Complex I (NADH:ubiquinone (UQ) oxidoreductase) is the first and the largest enzyme of the respiratory chain, catalysing the transfer of two electrons from NADH to UQ, coupled to the translocation of four protons across the bacterial or inner mitochondrial membrane. In bacterial complex I the 14 “core” subunits, necessary and sufficient for complex I function, are shared equally between the peripheral and membrane arms, together forming an L-shaped molecule. All known co-factors of complex I reside in the PA: the primary electron acceptor flavin-mononucleotide (FMN) is connected by the redox chain of seven Fe–S clusters to the quinone-binding site (Q-site) at the interface with the membrane domain. In this work we address this question by building and analyzing atomic structures of nine different conformational states of complex I, which were obtained by X-ray crystallography and single-particle cryo-EM.

In contrast, binding of DQ substrate to Q-site, in the absence of NADH or NAD+ in the NADH-binding site, promotes the rotation and tilt of the entire PA, including subunits Nqo4 and Nqo6 near Q-site, correlated with concerted changes in the region of the nearest proton pump, the E-channel. This suggests that motions near the Q-site can lead to changes in the E-channel and can be driven just by DQ binding, without any redox reaction. Other key residues, such as H384 from the key β1–β2 loop (33-QHPSTHG-39) in Nqo4 and M516, also contribute to the stabilization of the quinone ring, while secondary residues are involved specifically in the binding of each ligand. In particular, DQ interacts mainly with the residues mentioned above with its hydrocarbon chain surrounded by hydrophobic residues that complete the stabilization of the entire ligand. The presence of DQ in the Q-site significantly alters the conformation of the Nqo4 β-sheet, pulling β1–β2 loop (residues 32–39) about 1.5 Å inside the cavity towards DQ, allowing for stacking interactions between H384 and DQ. The opposite Nqo6 β-sheet also shifts in a similar direction, but the strand flanking the Q-cavity (P386 to F416) remains in place, thus effectively moving into the cavity and narrowing it. Therefore, as a result of DQ binding, the entire Q cavity undergoes conformational changes so that it “tightens” significantly around the quinone headgroup. Strikingly, this coupling was the strongest in the CXIDQ structure, because it was augmented by an additional edge, extending from the Nqo6 subunit. Despite the overall similarity of water networks, we identified one notable difference: only in the CXIDQ structure we observe the presence of a single water molecule nested between E32 and E67 of Nqo11 subunit. Thus, placement of water in this position leads to the formation of a unique continuous path extending from Nqo11 to Nqo14, that is, a path connecting the E-channel and the first antiporter.

>[2x]MTGPILSGLDPRFERTLYAHVGKEGSWTLDYYLRHGGYETAKRVLKEKTPDEVIEEVKRSGLRGRGGAGFPTGLKWSFMPKDDGKQHYLICNADESEPGSFKDRYILEDVPHLLIEGMILAGYAIRATVGYIYVRGEYRRAADRLEQAIKEARARGYLGKNLFGTDFSFDLHVHRGAGAYICGEETALMNSLEGLRANPRLKPPFPAQSGLWGKPTTINNVETLASVVPIMERGADWFAQMGTEQSKGMKLYQISGPVKRPGVYELPMGTTFRELIYEWAGGPLEPIQAIIPGGSSTPPLPFTEEVLDTPMSYEHLQAKGSMLGTGGVILIPERVSMVDAMWNLTRFYAHESCGKCTPCREGVAGFMVNLFAKIGTGQGEEKDVENLEALLPLIEGRSFCPLADAAVWPVKGSLRHFKDQYLALAREKRPVPRPSLWR;>[2x]MGFFDDKQDFLEETFAKYPPEGRRAAIMPLLRRVQQEEGWIRPERIEEIARLVGTTPTEVMGVASFYSYYQFVPTGKYHLQVCATLSCKLAGAEELWDYLTETLGIGPGEVTPDGLFSVQKVECLGSCHTAPVIQVNDEPYVECVTRARLEALLAGLRAGKRLEEIELPGKCGHHVHEVEV;>[2x]MVRVKVNDRIVEVPPGTSVMDAVFHAGYDVPLFCSEKHLSPIGACRMCLVRIGLPKKGPDGKPLLNEKGEPEIQWQPKLAASCVTAVADGMVVDTLSDVVREAQAGMVEFTLLNHPLDCPTCDKGGACELQDRTVEYGLYEKYYQKGPLELPVYTRFEFTRRHVDKHHPLSPFVILDRERCIHCKRCVRYFEEVPGDEVLDFIERGVHTFIGTMDFGLPSGFSGNITDICPVGALLDLTARFRARNWEMEETPTTCALCPVGCGITADTRSGELLRIRAREVPEVNEIWICDAGRFGHEWADQNRLKTPLVRKEGRLVEATWEEAFLALKEGLKEARGEEVGLYLAHDATLEEGLLASELAKALKTPHLDFQGRTAAPASLFPPASLEDLLQADFALVLGDPTEEAPILHLRLSEFVRDLKPPHRYNHGTPFADLQIKERMPRRTDKMALFAPYRAPLMKWAAIHEVHRPGEEREILLALLGDKEGSEMVAKAKEAWEKAKNPVLILGAGVLQDTVAAERARLLAERKGAKVLAMTPAANARGLEAMGVLPGAKGASWDEPGALYAYYGFVPPEEALKGKRFVVMHLSHLHPLAERYAHVVLPAPTFYEKRGHLVNLEGRVLPLSPAPIENGEAEGALQVLALLAEALGVRPPFRLHLEAQKALKARKVPEAMGRLSFRLKELRPKERKGAFYLRPTMWKAHQAVGKAQEAARAELWAHPETARAEALPEGAQVAVETPFGRVEARVVHREDVPKGHLYLSALGPAAGLRVEGRVLVPAGGEA;>[2x]MREEFLEEIPLDAPPEEAKELRTEVMTLNVGPQHPSTHGVLRLMVTLSGEEVLEVVPHIGYLHTGFEKTMEHRTYLQNITYTPRMDYLHSFAHDLAYALAVEKLLGAVVPPRAETIRVILNELSRLASHLVFLGTGLLDLGALTPFFYAFRERETILDLFEWVTGQRFHHNYIRIGGVKEDLPEEFVPELKKLLEVLPHRIDEYEALFAESPIFYERARGVGVIPPEVAIDLGLTGGSLRASGVNYDVRKAYPYSGYETYTFDVPLGERGDVFDRMLVRIREMRESVKIIKQALERLEPGPVRDPNPQITPPPRHLLETSMEAVIYHFKHYTEGFHPPKGEVYVPTESARGELGYYIVSDGGSMPYRVKVRAPSFVNLQSLPYACKGEQVPDMVAIIASLDPVMGDVDR;>MRLERVLEEARAKGYPIEDNGLGNLWVVLPRERFKEEMAHYKAMGFNFLADIVGLDYLTYPDPRPERFAVVYELVSLPGWKDGDGSRFFVRVYVPEEDPRLPTVTDLWGSANFLEREVYDLFGIVFEGHPDLRKILTPEDLEGHPLRKDYPLGETPTLFREGRYIIPAEFRAALTGKDPGLTFYKGGSRKGYRSLWADLKKAREVKG[2x];>[2x]MALKDLFERDVQELEREGILFTTLEKLVAWGRSNSLWPATFGLACCAIEMMASTDARNDLARFGSEVFRASPRQADVMIVAGRLSKKMAPVMRRVWEQMPDPKWVISMGACASSGGMFNNYAIVQNVDSVVPVDVYVPGCPPRPEALIYAVMQLQKKVRGQAYNERGERLPPVAAWKRTRG;>[2x]MSASSERELYEAWVELLSWMREYAQAKGVRFEKEADFPDFIYRMERPYDLPTTIMTASLSDGLGEPFLLADVSPRHAKLKRIGLRLPRAHIHLHAHYEPGKGLVTGKIPLTKERFFALADRAREALAFA;>[2x]MTLKALAQSLGITLKYLFSKPVTVPYPDAPVALKPRFHGRHVLTRHPNGLEKCIGCSLCAAACPAYAIYVEPAENDPENPVSAGERYAKVYEINMLRCIFCGLCEEACPTGAIVLGYDFEMADYEYSDLVYGKEDMLVDVVGTKPQRREAKRTGKPVKVGYVVPYVRPELEGFKAPTEGGKR;>MAPIQEYVGTLIYVGVALFIGVAALLVGALLGPKKPGRAKLMPYESGNDPAGEVKRFPVHFYVVAMLFILFDVEVAFLWPYAVSAGGLGLYGFLGVLAFTLLLFVGFLYEWWKGVMRWH[2x];>MTWSYPVDPYWMVALKALLVVVGLLTAFAFMTLIERRLLARFQVRMGPNRVGPFGLLQPLADAIKSIFKEDIVVAQADRFLFVLAPLISVVFALLAFGLIPFGPPGSFFGYQPWVINLDLGILYLFAVSELAVYGIFLSGWASGSKYSLLGSLRSSASLISYELGLGLALLAPVLLVGSLNLNDIVNWQKEHGWLFLYAFPAFLVYLIASMAEAARTPFDLPEAEQELVGGYHTEYSSIKWALFQMAEYIHFITASALIPTLFLGGWTMPVLEVPYLWMFLKIAFFLFFFIWIRATWFRLRYDQLLRFGWGFLFPLALLWFLVTALVVALDLPRTYLLYLSALSFLVLLGAVLYTPKPARKGGGA[2x];>MSLLEGLALFLLLLSGVLVVTLRNAIHAALALILNFLVLAGVYVALDARFLGFIQVIVYAGAIVVLFLFVIMLLFAAQGEIGFDPLVRSRPLAALLALGVAGILAAGLWGLDLAFTQDLKGGLPQALGPLLYGDWLFVLLAVGFLLMAATVVAVALVEPGKASRAKEAEKREEVAR[2x];>MSYLLTSALLFALGVYGVLTRRTAILVFLSIELMLNAANLSLVGFARAYGLDGQVAALMVIAVAAAEVAVGLGLIVAIFRHRESTAVDDLSELRG[2x];>MALLGTILLPLLGFALLGLFGKRMREPLPGVLASGLVLASFLLGAGLLLSGGARFQAEWLPGIPFSLLLDNLSGFMLLIVTGVGFLIHVYAIGYMGGDPGYSRFFAYFNLFIAMMLTLVLADSYPVMFIGWEGVGLASFLLIGFWYKNPQYADSARKAFIVNRIGDLGFMLGMAILWALYGTLSISELKEAMEGPLKNPDLLALAGLLLFLGAVGKSAQIPLMVWLPDAMAGPTPVSALIHAATMVTAGVYLIARSSFLYSVLPDVSYAIAVVGLLTAAYGALSAFGQTDIKKIVAYSTISQLGYMFLAAGVGAYWVALFHVFTHAFFKALLFLASGSVIHALGGEQDVRKMGGLWKHLPQTRWHALIGALALGGLPLLSGFWSKDAILAATLTYPFGGVGFYVGALLVAVLTAMYAMRWFVLVFLGEERGHHHPHEAPPVMLWPNHLLALGSVLAGYLALPHPLPNVLEPFLKPALAEVEAHHLSLGAEWGLIALSAAVALLGLWAGFVFFQRKVFPAWYLAFEAASREAFYVDRAYNALIVNPLKALAEALFYGDRGLLSGYFGLGGAARSLGQGLARLQTGYLRVYALLFVLGALLLLGVMRW[2x];>[2x]MVVLAVLLPVVFGALLLLGLPRALGVLGAGLSFLLNLYLFLTHPGGVAHAFQAPLLPGAGVYWAFGLDGLSALFFLTIALTVFLGALVARVEGRFLGLALLMEGLLLGLFAARDLLVFYVFFEAALIPALLMLYLYGGEGRTRALYTFVLFTLVGSLPMLAAVLGARLLSGSPTFLLEDLLAHPLQEEAAFWVFLGFALAFAIKTPLFPLHAWLPPFHQENHPSGLADALGTLYKVGVFAFFRFAIPLAPEGFAQAQGLLLFLAALSALYGAWVAFAAKDFKTLLAYAGLSHMGVAALGVFSGTPEGAMGGLYLLAASGVYTGGLFLLAGRLYERTGTLEIGRYRGLAQSAPGLAALALILFLAMVGLPGLSGFPGEFLTLLGAYKASPWLAALAFLSVIASAAYALTAFQKTFWEEGGSGVKDLAGAEWGFALLSVLALLLMGVFPGYFARGLHPLAEAFAKLLGGGA;>[2x]MTLAILAVFSVALTLLGFVLPPQGVKRATLLGLALALASLLLTWGKPFAFGPYAVDGVSQVFTLLALLGALWTVGLVRSGRFEFYLLVLYAALGMHLLASTRHLLLMLVALEALSLPLYALATWRRGQGLEAALKYFLLGALAAAFFLYGAALFYGATGSLVLGAPGEGPLYALALGLLLVGLGFKAALAPFHFWTPDVYQGSPTPVVLFMATSVKAAAFAALLRVAAPPEALALLVALSVVVGNLAALAQKEAKRLLAYSSIAHAGYMALALYTGNAQALGFYLLTYVLATGLAFAVLSQISPDRVPLEALRGLYRKDPLLGLAFLVAMLSLLGLPPLAGFWGKYLAFAEAARAGAWGVLVLALVTSAVSAYYYLGLGLAVFARPEETPFRPGPPWARAAVVAAGVLLLALGLLPGLVLPALAAGG;>MVRVGMRAAPRVSLEALKAALGGLKLSEAKVYLITDWQDKRDQARYALLLHTGKKDLLVPDAFGPAFPGGEEALSELVGLLLAQGARRFYEAVVSPGEMTALLDLPPEELLKRVMAIANPTDPGIYLKRAA[2x]Most extensively studied in this group are the F-specific filamentous phages (Ffs) that include viruses f1, fd and M13. Ffs are also strikingly simple—their single-stranded DNA genome encodes just 11 proteins, of which 5 form the phage capsid. pVIII is the major capsid protein that forms the filamentous body of the phage. The tips of the filament are formed of the minor capsid proteins which occur in pairs. pIII and pVI form the leading end of the infecting phage, which interacts with the host receptors to initiate entry, whereas pVII and pIX form the trailing end11,12.

The pointy tip is comprised of proteins pIII and pVI, present in 5 copies each. pIII is the largest and most structurally complex capsid protein. In our map, the N1-N2 domains and the glycine linkers are not visible, but density is seen for residues 257–404 of the C domain (accounting for the entire C domain minus the final two residues). The pIII C domain is comprised of several α-helices of differing lengths. Two β-strands form a hairpin loop which extends over the exterior of the main filamentous part of the virion; reminiscent of sepals protecting a flower bud (box 1 within Fig. 3a). We observed two cysteine residues (354 and 371) at the start and finish of the β-hairpin loop, in close enough proximity to form an intrachain disulphide bond. A disulphide bond in this position would pin the β-hairpin loop together and further reinforce the structural motif. pIII is predicted to contain three additional disulphide bonds; two in the N1 domain (between residues 7 and 36, and 46 and 53) and one in the N2 domain (between residues 188 and 201). The C-terminus of pIII is buried in the centre of the tip, where the 5 symmetry copies come together to form a distinct stricture in the virion lumen (box 2 within Fig. 3a). Density was observed for the entire pVI protein, which is composed of 3 α-helices arranged in a U shape. Five copies of each of the proteins are intertwined and arranged symmetrically to form the pointy tip. pIII makes 12 hydrogen bonds and 1 salt bridge with its two neighbouring pVI molecules. The outer surface of pVI (which is pIII-facing) is hydrophobic with two distinct rings of positive charge. pIII forms a negatively charged scaffold around it, with hydrophobic interactions being shielded at the centre of the assembled phage. Fatty acids were modelled into the map according to their size, suggesting one molecule of octanoic acid (C8) at the tip, followed by one molecule of butanoic acid (C4) and then 5 symmetry-related molecules of dodecanoic acid (C12) in the third site. Accessibility of lipids to detergent could explain the change in phage stability; in this case explaining why sarkosyl (with the larger head group compared to SDS) only affects the stability of the mutants with the largest truncations.

>[5x]MPVLLGIPLLLRFLGFLLVTLFGYLLTFLKKGFGKIAIAISLFLALIIGLNSILVGYLSDISAQLPSDFVQGVQLILPSNALPCFYVILSVKAAIFIFDVKQKIVSYLDWDK;>[5x]AETVESCLAKPHTENSFTNVWKDDKTLDRYANYEGCLWNATGVVVCTGDETQCYGTWVPIGLAIPENEGGGSEGGGSEGGGSEGGGTKPPEYGDTPIPGYTYINPLDGTYPPGTEQNPANPNPSLEESQPLNTFMFQNNRFRNRQGALTVYTGTVTQGTDPVKTYYQYTPVSSKAMYDAYWNGKFRDCAFHSGFNEDPFVCEYQGQSSDLPQPPVNAGGGSGGGSGGGSEGGGSEGGGSEGGGSEGGGSGGGSGSGDFDYEKMANANKGAMTENADENALQSDAKGKLDSVATDYGAAIDGFIGDVSGLANGNGATGDFAGSNSQMAQVGDGDNSPLMNNFRQYLPSLPQSVECRPFVFGAGKPYEFSIDCDKINLFRGVFAFLLYVATFMYVFSTFANILRNKES;>[35x]AEGDDPAKAAFDSLQASATEMIGYAWAMVVVIVGATIGIKLFKKFTSKAS> GRLVGLELSNFKSYRGVTKVGFGESNFTSIIGPNGSGKSNMMDAISFVLGVRSNHLRSNILKDLIYRGVLSNPQSAYVKAFYQKGNKLVELMRIISRNGDTSYKIDGKTVSYKDYSIFLENENILIKAKNFLVFQGDVEQIAAQSPVELSRMFEEVSGSIQYKKEYEELKEKIEKLSKSAEEKKILNQFLKIKKKRKELFEKTFDYVSDHL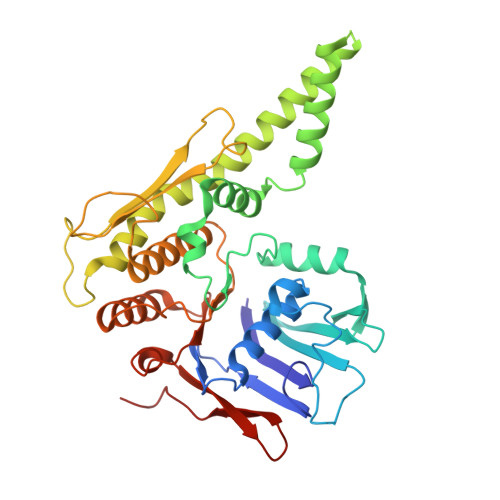DAIYRELTKNPNSNVELAGGNASLTIEDEDEPFNAGIKYHATPPLKRFKDMEYLSGGEKTVAALALLFAINSYQPSPFFVLDQVDAALDITNVQRIAAYIRRHRNPDLQFIVISLKNTMFEKSDALVGVYRQQQENSSKIITLDLSNYA2-{[(2S)-butan-2-yl]amino}-N-{(1R,2S)-1-hydroxy-3-phenyl-1-[(2R)-pyrrolidin-2-yl]propan-2-yl}-6-(methylsulfonyl)pyridine-4-carboxamide 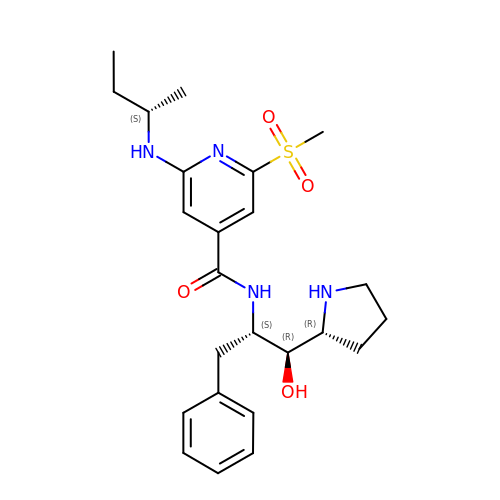| C24 H34 N4 O4 S | CNZLAHITQXPOEJ-YLTWVVNKSA-N>[12x]HHHHHHSEMTPREIVSELDKHIIGQDNAKRSVAIALRNRWRRMQLNEELRHEVTPKNILMIGPTGVGKTEIARRLAKLANAPFIKVEATKFTEVGYVGKEVDSIIRDLTDAAVKMVRVQAIEKNRYRAEELAEERILDVLIPPAKNNWGQTEQQQEPSAARQAFRKKLREGQLDDKEIEIDLAAAPMGVEIMAPPGMEEMTSQLQSM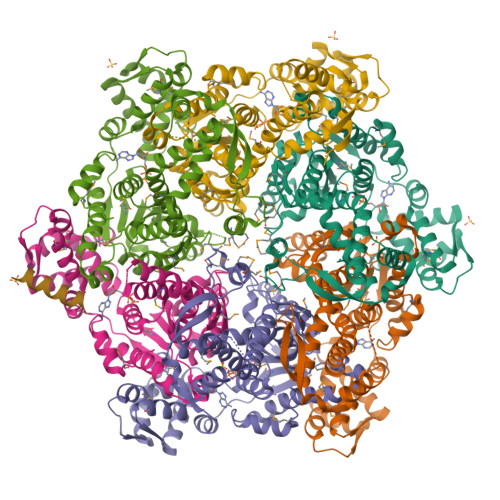FQNLGGQKQKARKLKIKDAMKLLIEEEAAKLVNPEELKQDAIDAVEQHGIVFIDEIDKICKRGESSGPDVSREGVQRDLLPLVEGCTVSTKHGMVKTDHILFIASGAFQIAKPSDLIPELQGRLPIRVELQALTTSDFERILTEPNASITVQYKALMATEGVNIEFTDSGIKRIAEAAWQVNESTENIGARRLHTVLERLMEEISYDASDLSGQNITIDADYVSKHLDALVADEDLSRFIL> MTDFLYSIFGLLILLGVLVTFHEWGHYWVAKKLGVKALRFSVGFGKPIWGRTNKHGTEFVIAPIPLGGYVRFVDEREGEVAEADLPFAFNRQQVWKRILIVLAGPMANFLLAIVVYAAVYMMGIAVGKPFVTNVLPNTVAAQANFPENSEILSVDGVQVKSLEDAIFAFVDHIDDDKTIKVVVKPLNQEPTTVVLDVSQWQEPDEGTIFDSLGLGFGRVNGEPSLGLVAKDSPAEKGGLKVGDTVVSVNGESISLWSEFVSFIENNPGKPLELIVARDGYQQPLVVTPEANERDRTIGYLGISPAFQGYNVINYGFFESFGKGAEQ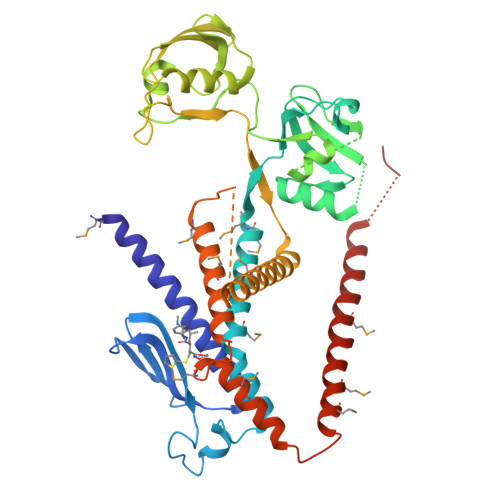TWVMVERIGSFLGKLITGKLSIKNLGGPVGIAQGAGQTAQAGMVAFLLYLAMISVNLGFVNLLPIPMLDGGHLMYYLVELVRGKPVSEKIMELGMRVGIILVLTIMAIALFFDINRINQLESSGENLYFQ>[3x]PFLELDTNLPANRVPAGLEKRLCAAAASILGKPADRVN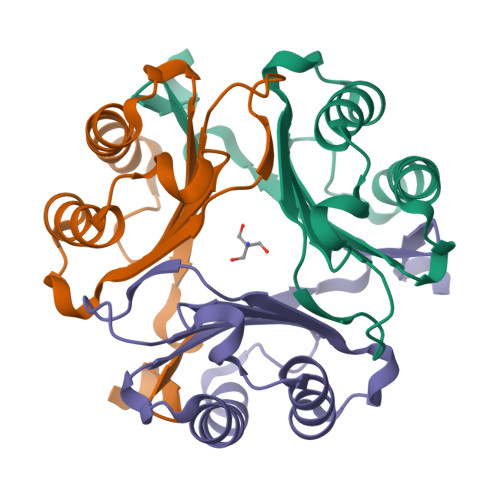VTVRPGLAMALSGSTEPCAQLSIASIGVVGTAEDNRSHSAHFFEFLTKELALGQDRILIRFFPLESWQIGKIGTVMTFL>GMSLPHLSSGEVASVLPLGKQLTQTPSAALFKEHRLEVMRMVLPAGKQVGSHSVAGPSTIQCLEGEVEIGVDGAQRRLHQGDLLYLGAGAAHDVNAITNTSLLVTV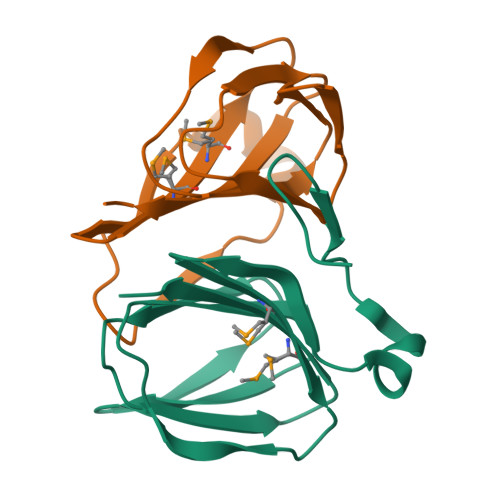VLVDRGGS[4x]>[2x]MNPKILIIGACGQIGTELTQKLRKLYGTENVIASDIRKLNTDVVNSGPFEVVNALDFNQIEHLVEVHKITDIYLMAALLSATAEKNPAFAWDLNMNSLFHVLNLAKAKKIKKIFWPSSIAVFGPTTPKENTPQYTIMEPSTVYGISKQAGERWCEYYHNIYGVDVRSIRYPGLISWSTPPGGGTTDYAVDIFYKAIA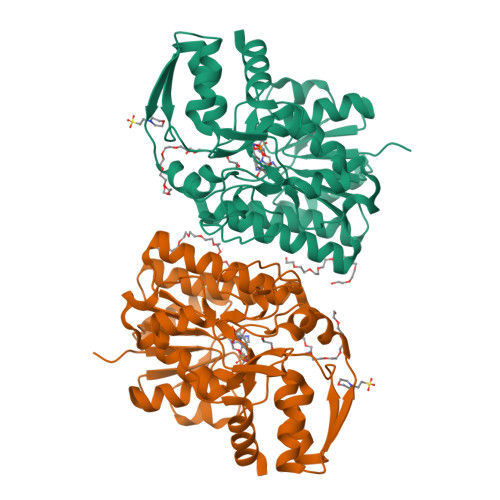DKKYECFLSSETKMPMMYMDDAIDATINIMKAPVEKIKIHSSYNLAAMSFTPTEIANEIKKHIPEFTITYEPDFRQKIADSWPASIDDSQAREDWDWKHTFDLESMTKDMIEHLS> TRPNHTIYINNLNEKIKKDELKKSLHAIFSRFGQILDILVSRSLKMRGQAFVIFKEVSSA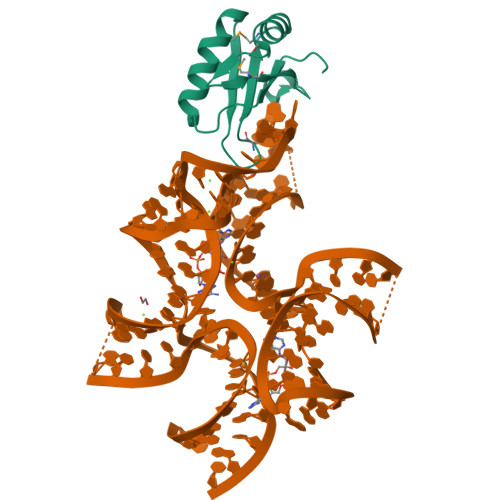TNALRSMQGFPFYDKPMRIQYAKTDSDIIAK>MDSTKAQTPEEQRAKNAKTILENIQIYERMCDLFGVSEDDKLIIENSISIERMIRVVTDKKYQDKKLKNAGSDPEKIANAGKVFCRLVESTAGKCSARLGMALKPNVEAVLTDVLGNELDRAAVLGKRMGFSAMFKSNLEEVLYQRGKNQLKKRNAAETFTLSQGASLEARFRPIMEKHLGVGTVVASIKNILASKKNGNYRNKMVRKPGGNRESWSPLEREISFLNKKLFPGPMRQLCKKFEYLNEQEKQLALNLMLDASLILKPQVTHKMIMPWSMWLAVKKYAEMNKGSPSLEDLAAYSGVRAFMAFNTACYMSKFTIGKGIVGDAEIMENGNDKMQTLAMACFGLAYEDTGIVAAMISQPMKKRYQLRVGNFNPPEKGTIKGTSAGYFHKWAEFGNRLPFNSFGTGESKQISNSGVFAVQRPSTTNIQRLAELMARNTGETSDNFTQLVQKIREQVGAFADQKAN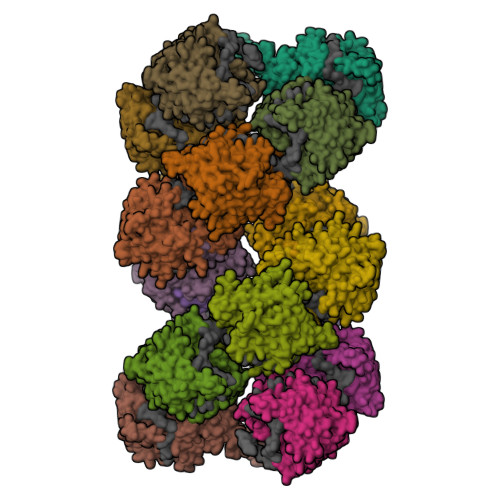LREFTGGYIYDITDVTKSNPKIPQLGGDSFFFEFTGSDVPRTGAKRRVGGADDVTPGTSQPKKRGRQGAGAESSMDIETVGED[16x]>[2x]MI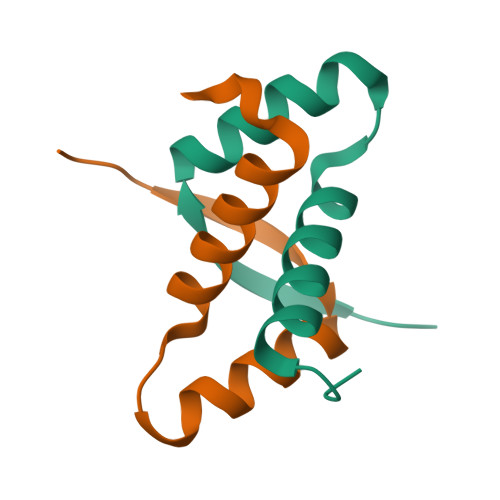VGNLGAQKAKRNDTPISAKKDIMGDKTVRVRADLHHIIKIETAKNGGNVKEVMDQALEEYIRKYLPDKL>MDNYQELAIQFAAQAVDRNEIEQWVREFAYQGFDARRVIELLKQYGGADWEKDAKKMIVLALTRGNKPRRMMMKMSKEGKATVEALINKYKLKEGNPSRDELTLSRVAAALAGRTCQALVVLSEWLPVTGTTMDGLSPAYPRHMMHPSFAGMVDPSLPGDYL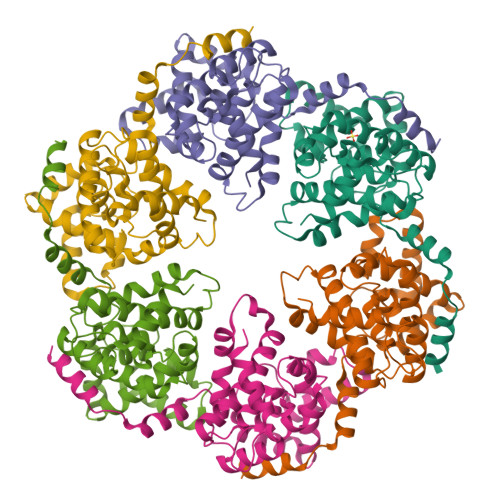RAILDAHSLYLLQFSRVINPNLRGRTKEEVAATFTQPMNAAVNSNFISHEKRREFLKAFGLVDSNGKPSAAVMAAAQAYKTAA[6x]> SRVDGGMSVTLHTDVGDIKIEVFCERTPKTCENFLALCASNYYNGCIFHRNIKGFMVQTGDPTGTGRGGNSIWGKKFEDEYSEYLKHNVRGVVSMANNGPNTNGSQ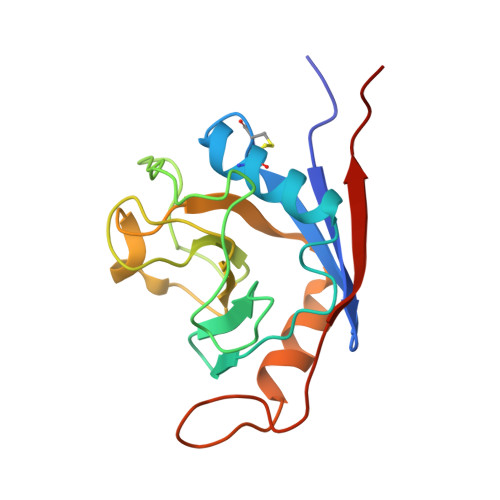FFITYGKQPHLDMKYTVFGKVIDGLETLDELEKLPVNEKTYRPLNDVHIKDITIHANPFAQ> MASFLKTI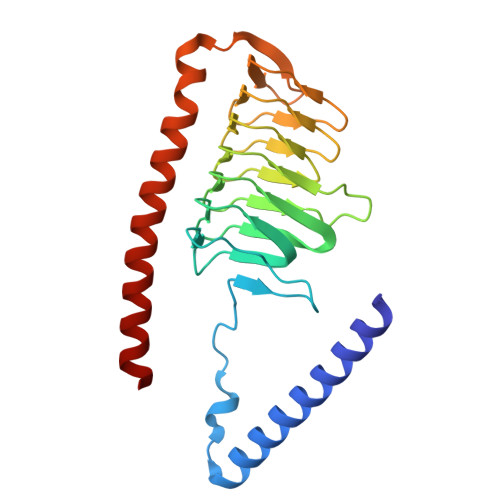VWRCGFAIKETGLALETLGCKLQGNYSFREKCSRHTPLTQYQFKAPSVGESTFVAPSALVSGDVIIGEKSSVLYNAVVRGEFKSVTIGEGSTISDNAYVGSSSEFSPETVIGSNVSVGSGAVLKGCTVGNNVLIGNNVIISEKATVEDNTILAPGSYVPEDVVVKSGELWSGSPAQKLRNLDEKELALFNTLSVGATELAADHAVIMKLLELKQKEFIK3-(3-phenylpropyl)-2-oxoglutarate | C14 H16 O5 | 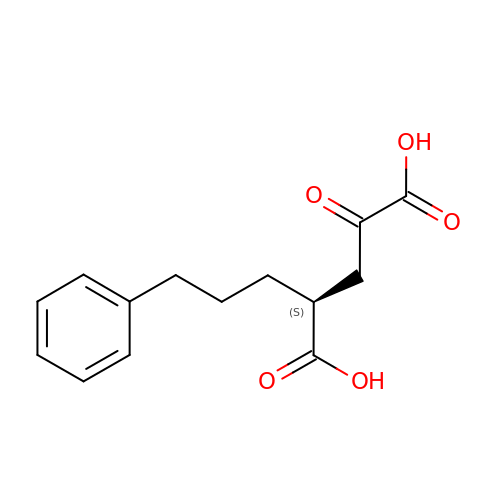JBXWROHAFLSAHP-NSHDSACASA-N(S,E)-3-HYDROXY-2-((3-HYDROXY-2-METHYL-5-(PHOSPHONOOXYMETHYL)PYRIDIN-4-YL)METHYLENEAMINO)-2-METHYLPROPANOIC 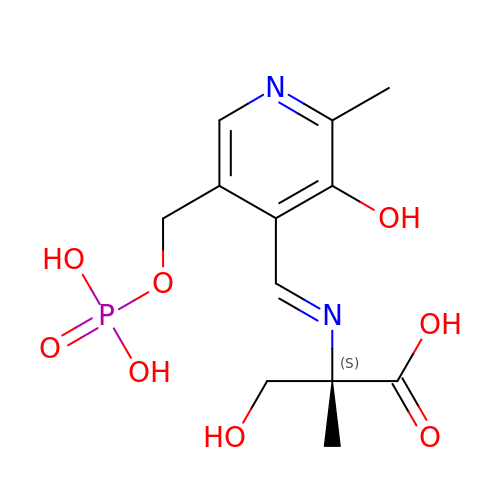ACID | C12 H17 N2 O8 P | ASXDVUDIJQGHKR-DRRTZOGYSA-N> PADFNGTWEMLSNDNFEDV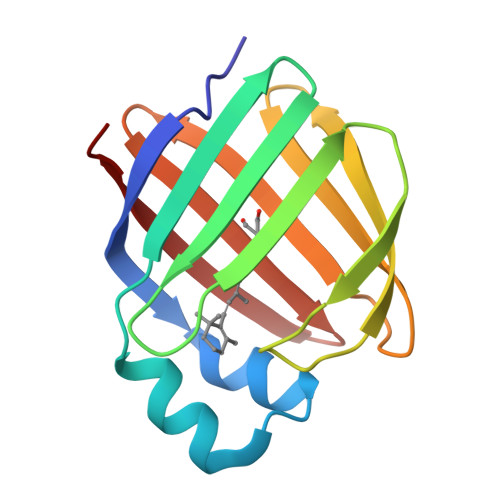MKALDIDFATRKIAVHLKQTKVIVQNGDKFETKTLSTFRNYEVNFVIGEEFDEQTKGLDNRTVKTLVKWDGDKLVCVQKGEKENRGWKQWIEGDLLHLEIHCQDKVCHQVFKKKN>MADPRTDNRNRKIPDAQVDAIKVPPHSLEAEQSVIGGLLLDNERWDTVSEHVMTQDFYSRPHRLIFDGVKSILEAGKPLDLITLSEYLEQREQLEDVGGFAYLADLAKNTPSAANINAYAEIVAERALVRNLIGVANEIADAGYDPQGRNAEDLLDLAESKVFAIAEARTSENEGPKNVDSILERTLERIELLYKTPQDGVTGVNTGFTDLNKKTAGLQGSDLIIVAARPSMGKTTFAMNLCENAAMEQDKPVLIFSLEMPAEQIMMRMLASLSRVDQTKIRTGQLDDEDWARISSTMGILMEKKNMYIDDSSGLTPTEVRSRARRIAREHGGLSLIMVDYLQLMRVPALTDNRTLEIAEISRSLKALAKELNVPVVALSQLNRSLEQRADKRPVNSD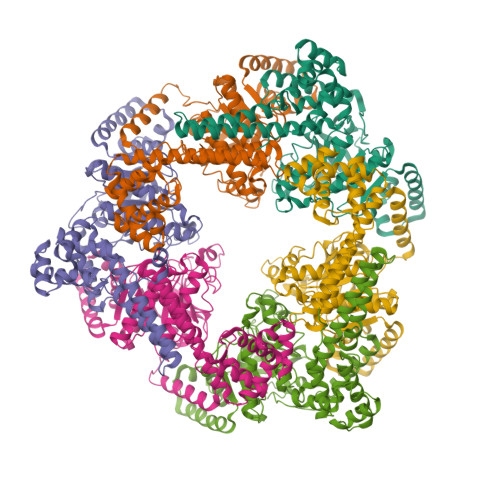LRESGSIEQDADLIMFIYRDEVYHPDSPLKGTAEIIIGKQRNGPIGSVRLTFQGHYSRFDNYAGPAFDDEHHHHHH[6x]> MARGLVIGEALIDIVDGPDPAEYVGGSPLNVAVGLARLGRDVDLLTHIGRDARGRRIAEYIESSGVQLVSGSQTADRTPTATARIGPDGSATYAFDLEWQIPDTPPVTPPLLVHTGSIAAAREPGCLAVAALLDAYRAAATVSFDPNVRPSLSADPDLTRERIQRLVERSD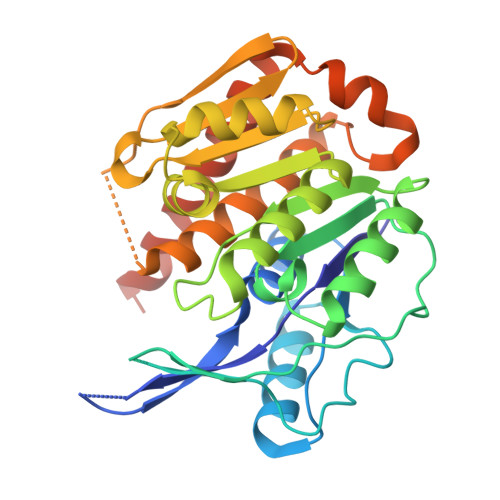IIKASAEDLHWIDPTQPPEQTARAWLACGPAIVALTLGDQGAVAFCAAGPASVPAQPVRVVDTVGAGDAFMAGLLDTLWEQGLLGADRRTELRKIGVSALTSALEVAALTSALTVARAGADLPYRADLRQSR(1S)-1-[(1P)-1-{6-[(3R)-3-(2-hydroxypropan-2-yl)pyrrolidin-1-yl]pyrimidin-4-yl}-1H-indazol-6-yl]spiro[2.2]pentane-1-carbonitrile | 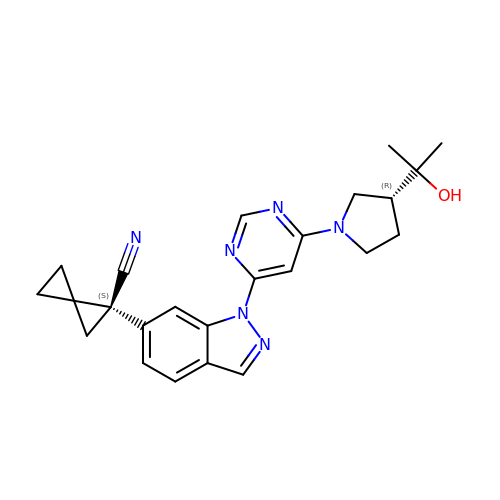C24 H26 N6 O | JCQABEJXHUSDMF-HOYKHHGWSA-N>MPSNCRRFEGKVAIVTAATKGIGLAIAERLLDEGASVVIGSRNQKNVDEAIEYLKNKGLTKVAGIAGHIASTDDQKKLVDFTLQKFGKINILVNNHGINPAFGHILEVSDQVWDKLFEVNVKAGFQMTKLVHPHIAKEGGGAIIFNASYSAYKSPPGIAAYGVTKTTLVGLTRALAMGLAKDNIRVNGIAPGVIKTKMSQV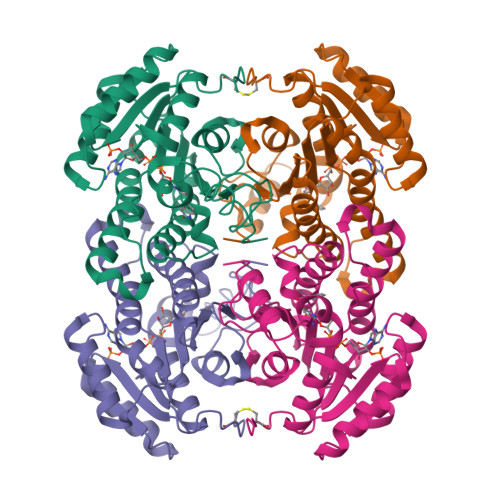LWDGGEDAEKELTDIQEIALGRLGVPDDCAGTVAYLASDDSSYITGEMIIIAGGVQARL[2x]tetradecylpropanedioic acid | 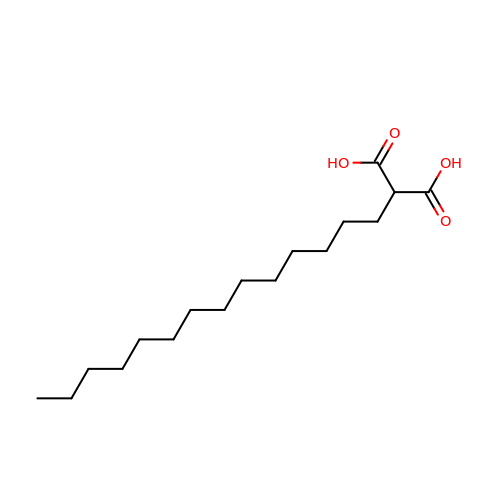C17 H32 O4 | SMTKGALBDOEZCA-UHFFFAOYSA-N> VRSSSRTPSDMPVAHVVANPQAEGQLQWLNRRANALLANGVELRDNQLVVPSEGLYLIYSQVLFSGQGCPSTHVLLTHTISRIA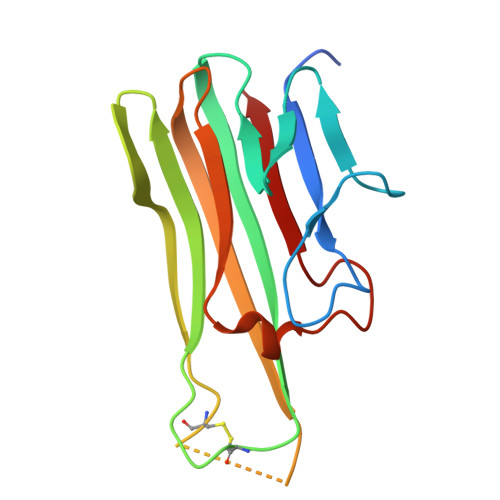VSYQTPVNLLSAIRSPCQRETPEGAEANPWYEPIYLGGVFQLEPGDRLSAEINRPDYLDFAESGQVYFGIIAL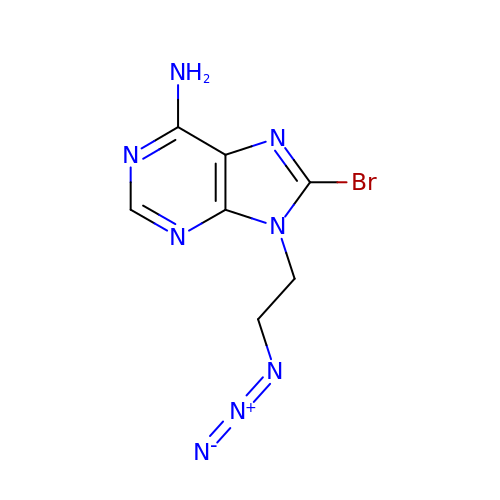9-(2-azidoethyl)-8-bromanyl-purin-6-amine | C7 H7 Br N8 | LMIPSSRPSGTFEB-UHFFFAOYSA-N>AVVRFVFRGDLAELMLRAVKDHLKKEGPHWNITSRGNELVVRGIHESDAKRIQKE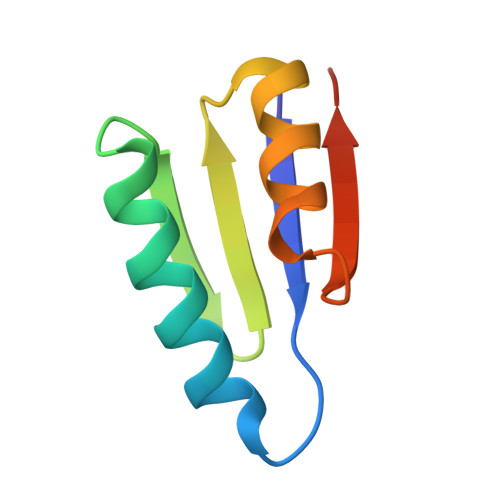FPSVQSTIQAAAAAA[12x]>[2x]GUACACGACAAUAC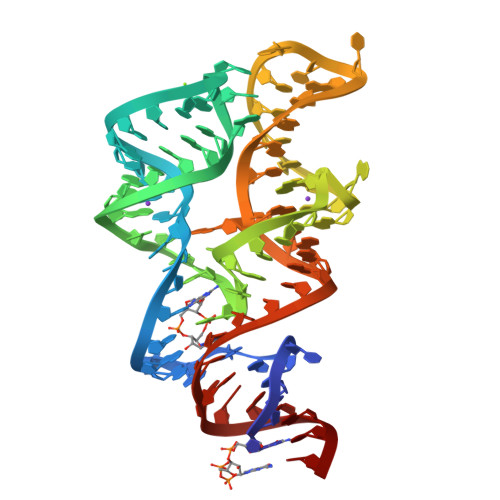UAAACCAUCCGCGAGGAUGGGGCGGAAAGCCUAAGGGUCUCCCUGAGACAGCCGGGCUGCCGAAAUAUC> MVNILWELLHNMRDHYNEVLLQRWVHVFREILDKEQFLPMVVQNT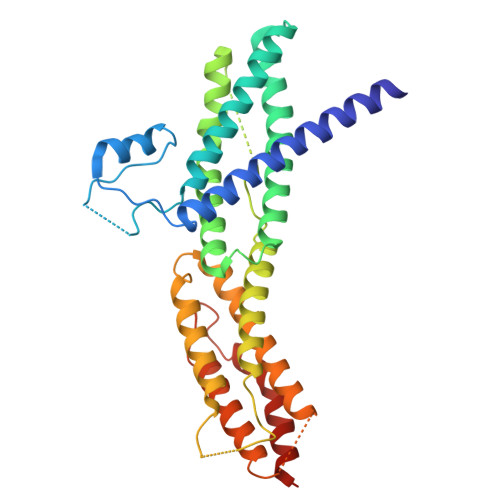EEYECIIERFPFHSEQLENAPFPKKFPFSRMVPEVYHQAKEFMYACMKFAEELTLSPNEVAAMVRKAANLLLTRSFSGCLSVVFRQPSITLTQLIQIIIDTQYLEKAGPFLDEFVCHMTNTERSVSQTPSAMFHVARQDAEKQVGLRICSKIDEFFELSAYDWLLVEPPGIASAFITDMISYLKSTFDSFAFKLPHIAQAACRRTFEHIAEKIYSIMYDEDVKQISTGALTQINLDLMQCEFFAASEPVPGLKEGELSKYFLRNRQLLDLLILEHHHHHH> SMRSSSHSSRRAKSVEDDAEGHLIYHVGDWLQERYEIVSTLGEGTFGRVVQCVDHRRGGARVALKIIKNVEKYKEAARLEINVLEKINEKDPDNKNLCVQMFDWFDYHGHMCISFELLGLSTFDFLKDNNYLPYPIHQVRHMAFQLCQAVKFLHDNKLTHTDLKPENILFVNSDYELTYNLEKKRDERSVKSTAVRVVDFGSATFDHEHHSTIVSTRHYRAPEVILELGWSQPCDVWSIGCIIFEYYVGFTLFQTHDNREHLAMMERILGPIPSRMIRKTRKQKYFYRGRLDWDENTSAGRYVRENCKPLRRYLTSEAEEHHQLFDLIESMLEYEPAKRLTLGEAL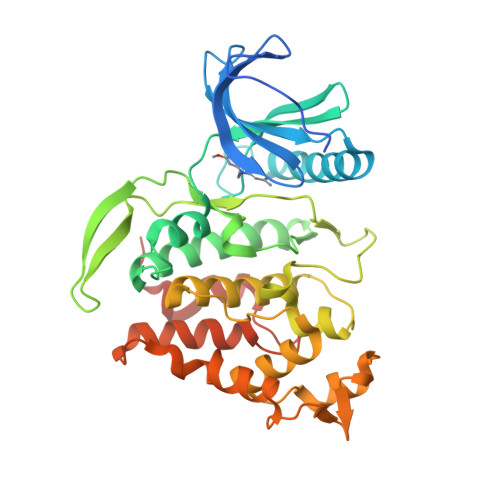QHPFFARLRAEPPNKLWDSSRD1,3-benzothiazol-6-amine | C7 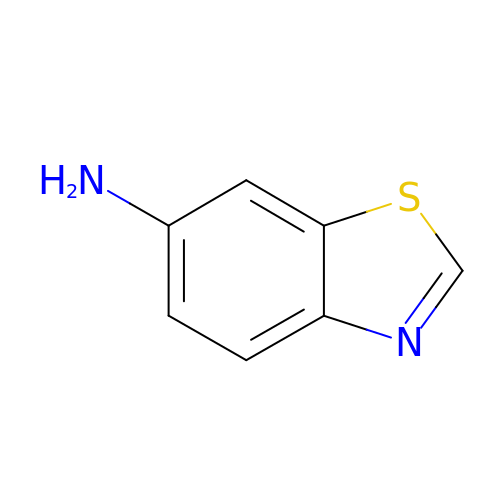H6 N2 S | FAYAYUOZWYJNBD-UHFFFAOYSA-N> MEELKEIMKSHILGNPVRLGIMIFLLPRRKAPFSQIQKVLDLTPGNLDSHIRVLERNGLVKTYKVIADRPRTV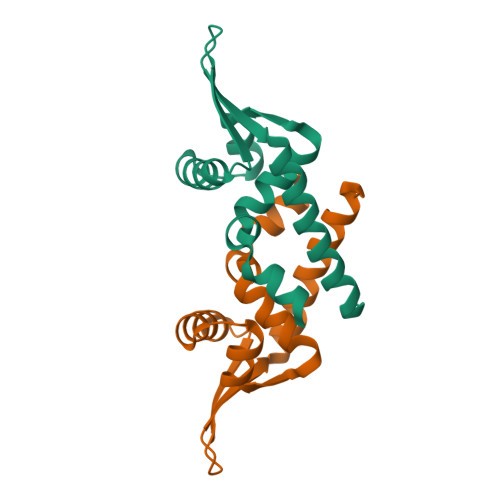VEITDFGMEEAKRFLSSLKAVIDGLDL> MPAKAAAKPVKPATKAAPKPANKAPAPKAAAAKPVAKAAPKAAAPAVRPASGSSNGVYVKNWGTGSVADATN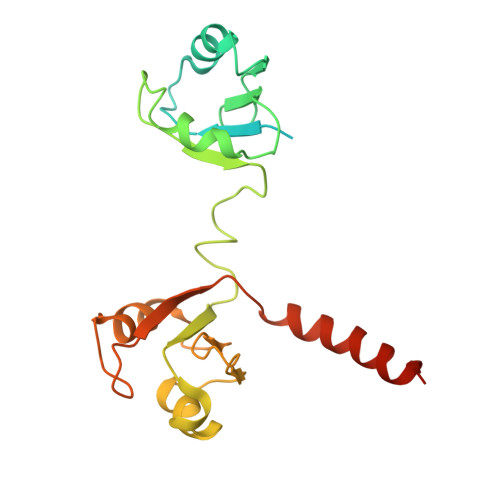VFSAAGKVVKVQLRRQRYALVFFENSAAVKKAIDLFNEKEVLGQTVLVVPAKASPKPDAHENSSCVFVSPIFRPSTTKAQVMELFAGVKVQRLRMYRQNFAYAYLDSPAAAKKFVEEKNGTAFRGHTLRVALSARSLEKLRARQEVANVVIAAHRHYKVHERQ> SRVLLALHDRAPQLKISDDRLTVVGEKGYSMVRASHGVRKGAWYFEITVDEMPPDTAARLGWSQPLGNLQAPLGYDKFSYSWRSKKGTKFHQSIGKHYSSGYGQGDVLGFYINLPEDTISGRGSSEIIFYKNGVNQGVAYKDIFEGVYFPAISLYKSCTVSINFGPCFKYPPKDLTYRPMSDMG;> ARTKQTARK;> SDLPMPMRFRHLKKTSKEAVGVYRSPIHGRGLFCKRNIDAGEMVIEYAGIVIRSILTDKREKYYDSKGIGSSYMFRIDDSEVVDATMHGNAARFINHSCEPNCYSRVINIDGQKHIVIFAMRKI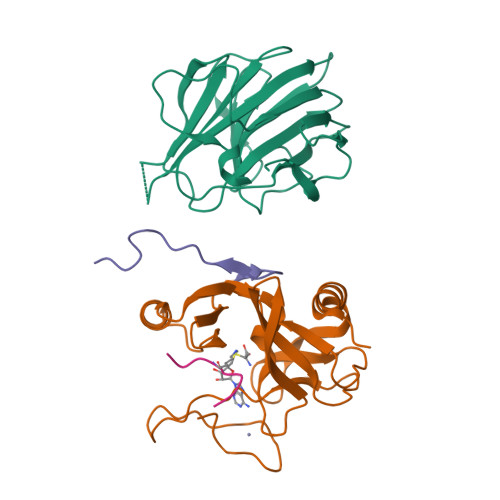YRGEELTYDYKFPIEDASNKLPCNCGAKKCRKFLN;> SAFAPDFKELDENVEYEERESEFDIED>[2x]T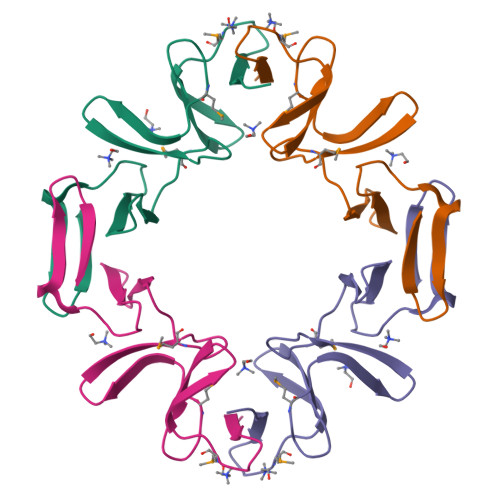DGNWYWFDNSGEMATGWKKIADKWYYFNEEGAMKTGWVKYKDTWYYLDAKEGAMVSNAFIQSADGTGWYYLKPDGTLADRPEFTVEPDGLITVK5-methyl-2-piperidin-4-yl-6-pyridin-4-yl-pyridazin-3-one 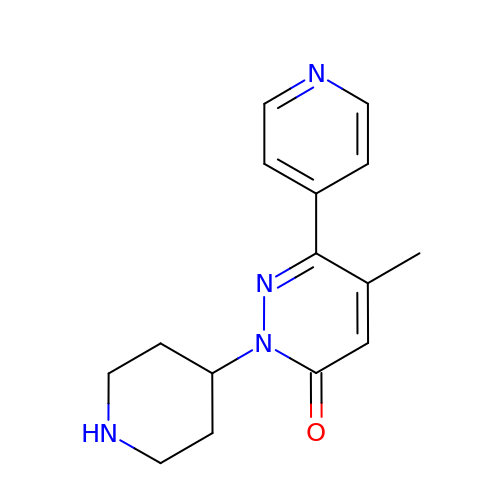| C15 H18 N4 O | DDBCCLBDEPERNR-UHFFFAOYSA-N>[2x]SKAALSEEELEKKSKAIIEEYLHLNDMKEAVQCVQELASPSLLFIFVRHGVESTLERSAIAREHMGQLLHQLLCAGHLSTAQYYQGLYEILELAEDMEIDIPHVWLYLAELVTPILQEGGVPMG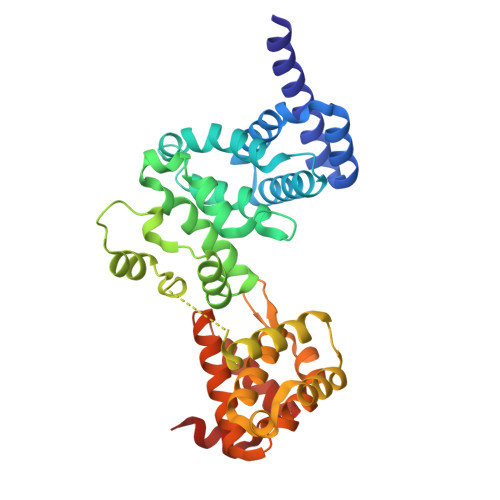ELFREITKPLRPLGKAASLLLEILGLLCKSMGPKKVGTLWREAGLSWKEFLPEGQDIGAFVAEQKVEYTLGEESEAPGQRALPSEELNRQLEKLLKEGSSNQRVFDWIEANLSEQQIVSNTLVRALMTAVCYSAIIFETPLRVDVAVLKARAKLLQKYLCDEQKELQALYALQALVVTLEQPPNLLRMFFDALYDEDVVKEDAFYSWESSKDPAE> AMADIGSEMKEYDVFIIGSGMAGMTIANKCASKGLTVGITDELPYGGTCALRGCDPKKVIIGATEVRDFAKRLKGSGIDTIPKVNWKDIMAFKQSFVDEMPPKVEKGYKRNGIDTFHSSAKFLSQNTLEIGNEKIKAKKIVIASGSKPRVLEFEGGHFAKTSADFLNLDELPKSLLFIGGGYIAFEFAHIAARCGAEVTIVHRGNNPLENFEQDIVKHLVSATKKLGVKLILNTDVTAIEKADKKFRVKGKSAEKTEYFEAEAVFNSAGRPPAIFDLELEKAGISFTKKGVSVNEHLQNTSNPIVYAAGDAADSEGLPLTPVAVLEGHTVASNIIKGNHKKISYPPMPTVVFTLPTMASVGYTESRARELNYNIQVNYKEVGDWFNAKRLNVAEYAFKTIIDEETQTILGAHLIGPHTEETINLFAMAIKTKMKVNDIRTMIFSYPTLASDIPHML

In this study, we identified and characterized mercuric reductase (GbsMerA), which is coded as a component of the mercury resistance (mer) operon in G. salicanalis isolated from Antarctic soil. We characterized GbsMerA, a mercury reductase belonging to the mercury-resistant operon of Gelidibacter salicanalis PAMC21136, and found its maximum activity of 474.7 µmol/min/mg in reducing Hg+2. As seen in the structures of thioredoxin reductase (high Mr), trypanothione reductase, glutathione reductase, glutathione amide reductase, and dihydrolipoamide dehydrogenase, the overall structure of GbsMerA also comprises an FAD-binding domain (residues 1–146), an NADPH-binding domain (residues 147–275), an interface domain (residues 276–340), and a dimerization domain (residues 341–447)29. GbsMerA has two pathways that connect molecular surfaces to the si- and re-faces of the isoalloxazine ring in FAD.

Furthermore, we determined the GbsMerA–NADPH complex structure. Residues at the NADPH-binding site are conserved, similar to those found in other MerAs, and generate positively charged surfaces. These residues included Arg141, His194, Arg195, and the nitrogen atoms of glycines (G171, and G173). Structural comparison between the FAD- and FAD–NADPH-bound forms indicated that these residues were not changed upon NADPH binding, except for Tyr174 and Arg195. Arg195, which is located at the edge of the central sheet of the NAPDH domain, was tilted toward the solvent area in the NADPH complex. Another residual change observed upon NADPH binding was Tyr174. However, in the NADPH complex, the side chain of Tyr174 was flipped opposite to the isoalloxazine ring of FAD by 6.5 Å (OH group). The Tyr174 residue was replaced with the nicotinamide ring of NADPH. Therefore, the isoalloxazine ring of FAD, nicotinamide ring of NAPDH, and Tyr174 are aligned and stacked with cation–π interaction. Mutation of Tyr174 to Phe showed decreased activity by 50%, indicating that the interaction of Tyr174 with the isoalloxazine ring of FAD through the hydroxyl group of tyrosine may be important for controlling the NADPH binding.>[2x]DYDYGTDTCPFPVLANKTNKAKFVGCHQKCNGGDQKLTDGTACYVVERKVWDRMTPMLWYEC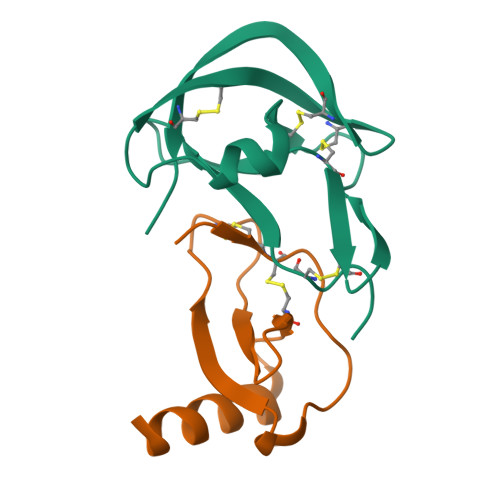PLGECKNGVCEDLRKKEDCRKGN;>[2x]ARGTNVGRECCLEYFKGAIPLRKLKTWYQTSEDCSRDAIVFVTVQGRAICSDPNNKRVKNAVKYLQSLERS> MIIPALDLIGGTVVRLHQGDYARQRDYGNDPLPRLQD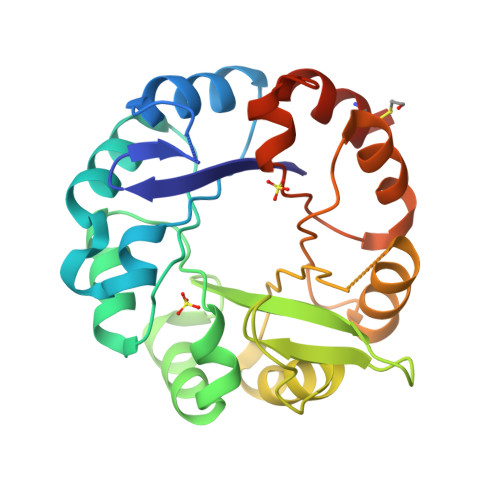YAAQGAGVLHLVDLTGAKDPAKRQIPLIKTLVAGVNVPVQVGGGVRTEEDVAALLKAGVARVVIASTAVKSPDVVKGWFERFGAQALVLALDVRIDEHGTKQVAVSGWQENSGVSLEQLVETYLPVGLKHVLCTDISRDGTLAGSNVSLYEEVCARYPQIAFQSSGGIGDIDDIAALRGTGVRGVIVGRALLEGKFTVKEAIQCWQNVKGHHHHHH2-amino-1H-benzimidazol-7-ol | C7 H7 N3 O | 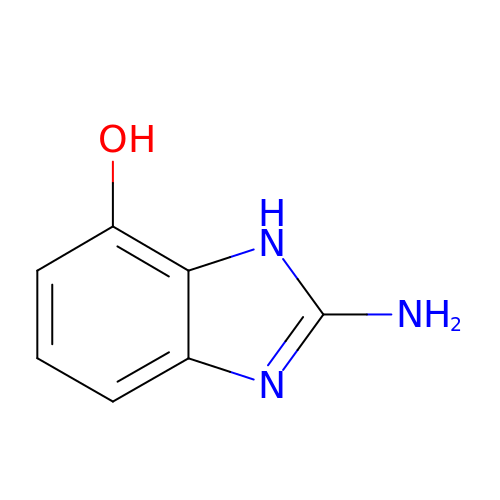BBSYMXYQDPASMX-UHFFFAOYSA-N> PKRELEQGVAFSDLCNFLVTPTVQGWKVYWAGLEFDVNQKGITLLNRLKVNDFAPAWAMTRNLFPHLFKNQQSEVQTPIWALRVILAAG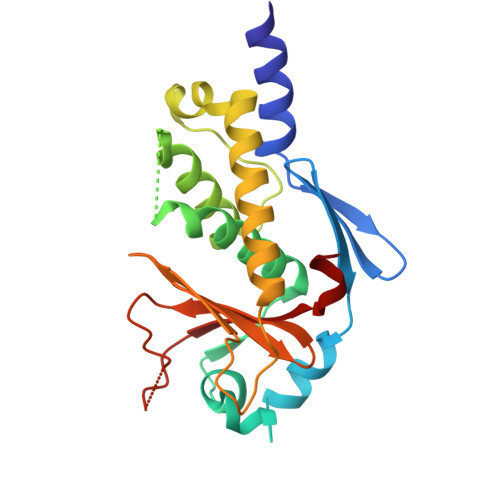ILDQLMDHSLIEPLSGALNLIADWLLTTSTNHFNMRTQRVKDQLSMRMLSLIRSNIINFINKLETLHVVNYKGLLSSVEIGTPSYAIIITRTNMGYLVEVQEPDKSAMDIRHPGPVKFSLLHESTLK> SSIYARGRGGSSTDQPVANPYNTKEISLAAGLVQQTYCDSTENGLKIGDSELLYTMGEGYARQRVNIYHSPSLGIAVAIEGTNLFSLNSDLHDAKFWQEDPNERYIQYYPKGTKLMHGFQQAYNDLMDDIFTAVKKYKKEKNEKRVTVIGHSLGAAMGLLCAMDIELRMDGGLYKTYLFGLPRLGN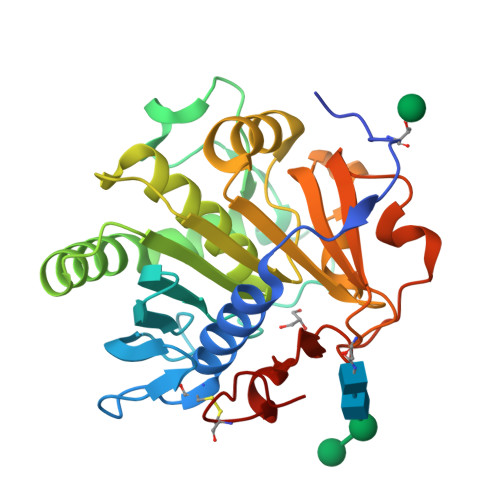PTFASFVDQKIGDKFHSIINGRDWVPTVPPRALGYQHPSDYVWIYPGNSTSAKLYPGQENVHGILTVAREFNNDDHQGIYFHTQIGAVMGECPAQVGAH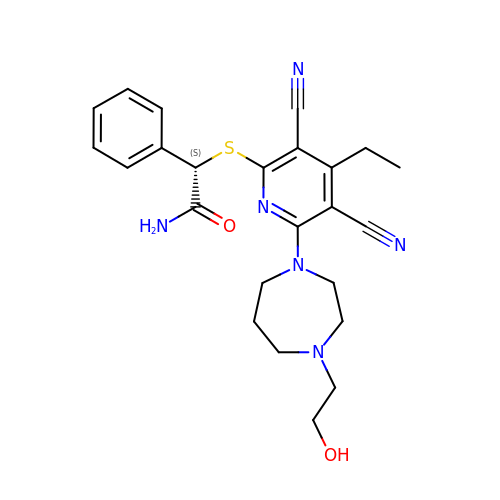(2S)-2-({3,5-dicyano-4-ethyl-6-[4-(2-hydroxyethyl)-1,4-diazepan-1-yl]pyridin-2-yl}sulfanyl)-2-phenylacetamide | C24 H28 N6 O2 S | IHXXDZHXEBKTKE-NRFANRHFSA-N1-[(2R)-2-[(4-chlorobenzyl)oxy]-2-(2,4-dichlorophenyl)ethyl]-1H-imidazole 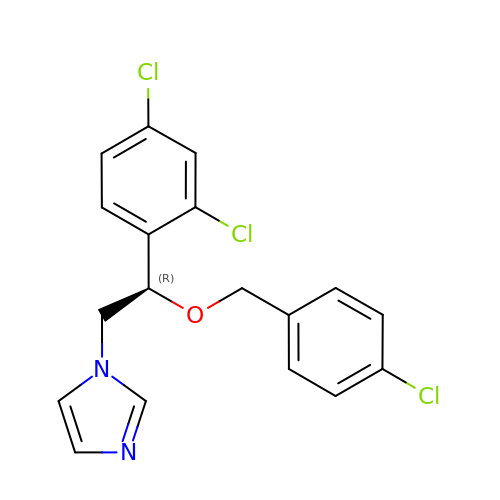| C18 H15 Cl3 N2 O | LEZWWPYKPKIXLL-SFHVURJKSA-N> MGKKQTQRNVFRCNVIGVKNCGKSGVLQALLGRNLMRQKKIREDHKSYYAINTVYVYGQEKYLLLHDISESEFLTEAEIICDVVCLVYDVSNPKSFEYCARIFKQHFMDSRIPCLIVAAKSDLHEVKQEYSISPTDFCRKHKMPPPQAFTCNTADAPSKDIFVKLTTMAMYPHVTQADLKSSTFLEHHHHHH

Human Miro1 and Miro2 (hMiro1, hMiro2, also called RhoT1 and RhoT2) are MOM protein homologs that play a critical role in mitochondrial trafficking38394041424344. Both associate with Parkin upon mitochondrial depolarization and are ubiquitinated on multiple lysines18374546. Here, we demonstrate that the cGTPase domain is necessary and sufficient for efficient ubiquitination of either hMiro1 or hMiro2 by p-S65 Parkin. We also find that despite considerable similarities between these two substrates, Parkin modifies hMiro1 much more robustly than hMiro2.

To better understand the difference in ubiquitination efficiency between hMiro1 and hMiro2, we first determined the crystal structures of the isolated cGTPase domains of both proteins to high resolution (hMiro1-C: 2.25 Å; hMiro2-C: 1.69 Å). Unexpectedly, both domains crystallized as symmetric dimers. The dimer interface is a highly conserved hydrophobic surface along one face of the cGTPase domain, which, in the intact hMiro1-BC structure, forms the interface with the second hidden EF hand (hEF2). The cGTPase does not mediate dimerization in the context of the full-length molecule, as the hEF2/cGTPase interface is mutually exclusive with cGTPase dimerization, and hMiro1-BC is purely monomeric even at high concentrations. Interestingly, although the same conserved residues mediate dimerization in hMiro1-C and hMiro2-C, their dimer relationships differ significantly. We performed size exclusion chromatography with in-line multi-angle light scattering (SEC-MALS) and confirmed that both hMiro1-C and hMiro2-C dimerize in solution. Subsequently, we successfully disrupted dimerization of hMiro1-C in solution by introducing three mutations at the hydrophobic interface (V418R, Y470S, L472A), thereby generating a stable hMiro1 cGTPase monomer (hMiro1-CM). We note that the two lysines in addition to K572 identified as ubiquitinated by mass spectrometry of the hMiro1-CD, K454 and K512, can be mapped in the dimer, but not the monomer, to roughly the same continuous surface containing K572.> ATCTVKSVDDAKDIAGCSAVTLNGFTVPAGNTLVLNPDKGATVTMAGDITFAKTTLDGPLFTIDGTGINFVGADHIFDGNGALYWDGKGTNNGTHKPHPFLKIKGSGTYKKFEVLNSPAQAISVGPTDAHLTLDGITVDDFAGDTKNLGHNTDGFDVSANNVTIQNCIVKNQDDCIAINDGNNIRFENNQCSGGHGISIGSIATGKHVSNVVIKGNTV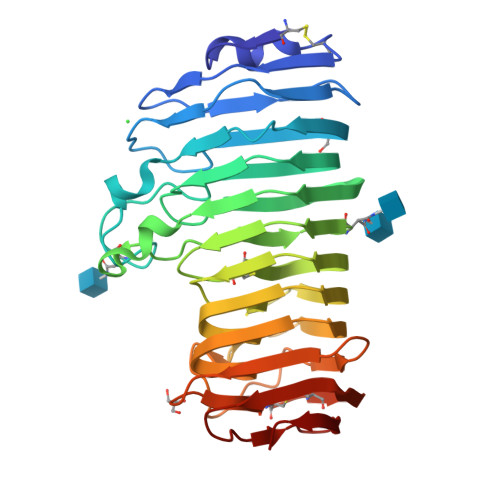TRSMYGVRIKAQRTATSASVSGVTYDANTISGIAKYGVLISQSYPDDVGNPGTGAPFSDVNFTGGATTIKVNNAATRVTVECGNCSGNWNWSQLTVTGGKAGTIKSDKAKITGGQYL> MSKLELLPAVDVRDGQAVRLVHGESGTETSYGSPLEAALAWQRSGAEWLHLVDLDAAFGTGDNRALIAEVAQAMDIKVELSGGIRDDDTLAAAL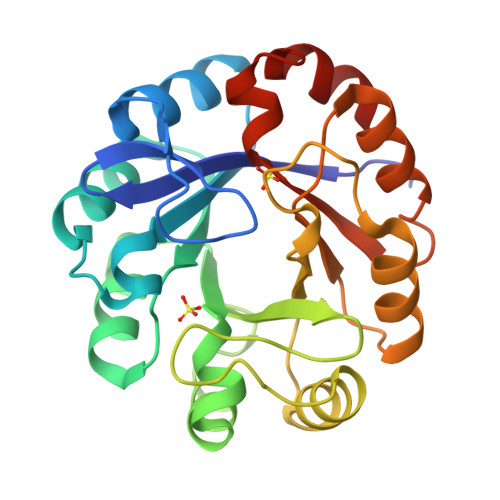ATGCTRVNLGTAALETPEWVAKVIAEHGDKIAVGLDVRGTTLRGRGWTRDGGDLYETLDRLNKEGCARYVVTDIAKDGTLQGPNLELLKNVCAATDRPVVASGGVSSLDDLRAIAGLVPAGVEGAIVGKALYAKAFTLEEALEATSLEPG4-[[3-[2-chloranyl-6-(trifluoromethyl)phenyl]-5-(1~{H}-pyrazol-4-yl)-1,2-oxazol-4-yl]methoxy]benzoic acid | C21 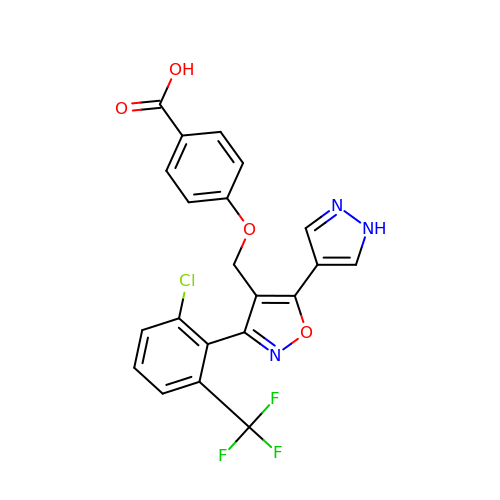H13 Cl F3 N3 O4 | OPIGXBQPAXXYLU-UHFFFAOYSA-N>MVAKEWQENKSWNAHFTEHKSQGVVVLWNENKQQGFTNNLKRANQAFLPASTFKIPNSLIALDLGVVKDEHQVFKWDGQTRDIATWNRDHNLITAMKYSVVPVYQEFARQIGEARMSKMLH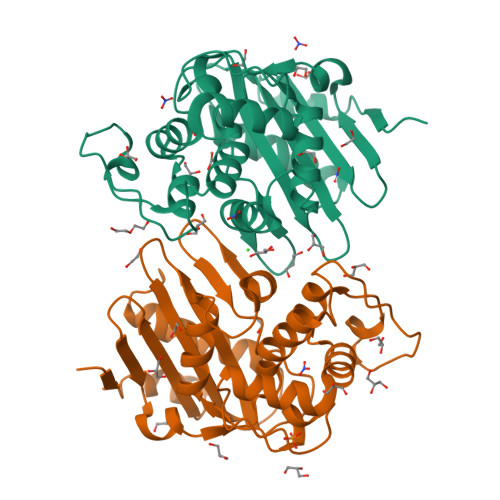AFDYGNEDISGNVDSFWLDGGIRISATEQISFLRKLYHNKLHVSERSQRIVKQAMLTEANGDYIIRAKTGYSTRIEKIGWWVGWVELDDNVWFFAMNMDMPTSDGLGLRQAITKEVLKQEKIIPFEHHHHHHHH[2x]>[2x]GSMGKPFFTRNPSELKGKFIHTKLRKSSRGFGFTVVGGDEPDEFLQIKSLVLDGPAALDGKMETGDVIVSVNDTCVLGHTHAQVVKIFQSIPIGASVDLELCRGYPLGSSAYGSVKAYTNFDAERDALNIETAIKTKGVDEVTIVNILTNRSNEQRQDIAFAYQRRTKKELASALKS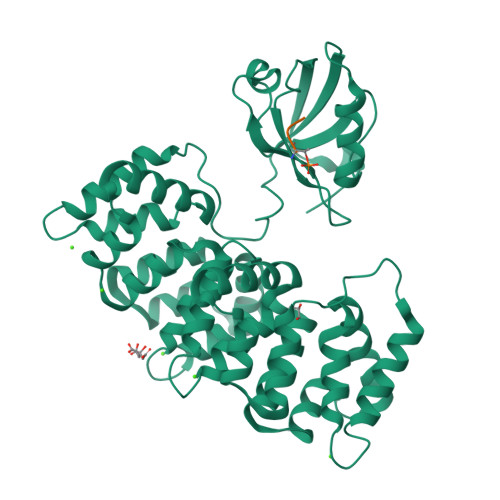ALSGHLETVILGLLKTPAQYDASELKASMKGLGTDEDSLIEIICSRTNQELQEINRVYKEMYKTDLEKDIISDTSGDFRKLMVALAKGRRAEDGSVIDYELIDQDARDLYDAGVKRKGTDVPKWISIMTERSVPHLQKVFDRYKSYSPYDMLESIRKEVKGDLENAFLNLVQCIQNKPLYFADRLYDSMKGKGTRDKVLIRIMVSRSEVDMLKIRSEFKRKYGKSLYYYIQQDTKGDYQKALLYLCGGDD;>SSRTRRETQL[2x]>VSFRQKRTRIPLLAMTVTALAAAVCGVTTAPAATGAEVAVPLSVGAAAGNATPIPGYVIQSSAQVSDDSAVSKPGFPTSGWYPVSSRSTVYAGLLQNGKYADPFYSTNMQNVPAAQFSVPWWYRTDLNVDDTSSRTYLDFSGVLSKADVWVNGTKVATKDQVNGAYTRHDLDITAQVHTGVNSVAFKVYPNDPNRDLSMGWIDWAQTPPDQNMGIVRDVLVRRSGAVALRSAHVIQKLNSALDHADLTVKADVRNDSANAVQTTVAGTVAGKPISQTVSLAAKERKTVTFPLVGLDRPNVWWPAGMGGQHRYDLDLTASVGGTPSDAAKSKFGVRDVKATLNSSGGRQYSVNGKPLLIRGGGYTPDLFLRWNETAAADKLKYVLNLGLNTVRLEGHIEPDEFFDIADDLGVLTMPGWECCDKWEGQVNGEEKGEPWVESDYPIAKASMFSEAERLRDHPSVISFHIGSAFAPDRRIEQGYLDAMKAADFLLPVIPAASARPSPITGASGMKMNGPYDYVPPVYWYDKSQKDRGGAWSFNSETSAGVDIPTMDTLKRMMSASELDTMWKNPSAKQYHRSSSDTFGNLKLFGDALTKRYGASANLNDFVRKAQLSQYENVRAEFESHSRNYTDSTNPSTGLIYWMLNSPWTSLHWQLFDAYMDQNGAYYGAKKANEPLHIQYSHDNRSVVVINQTSNAVSGLTATTKLYNLDGTEKYSNTKTGLSVGALGAKATAVTVPAVSGLSTTYLAKNVLTDSSGKEVSRNVYWLSTKADTLNWGGSDWYYTPQSAF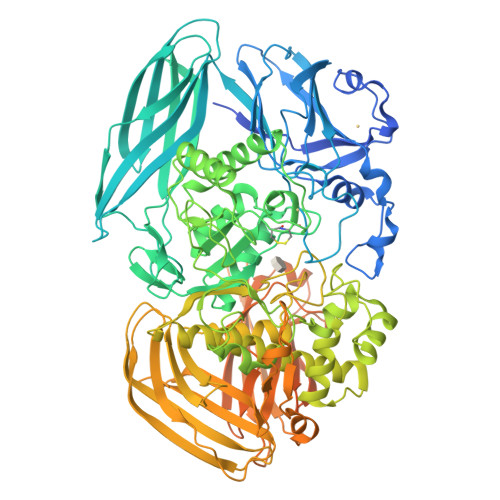ADLSGLNNLGQSAVGATANSVAGADGTTTTTVTLKNTSGGRLPAFYVDSKVVDSAGKPVLPVEWNANAVSLWPGETTTLTAKYRTADLKGSKPSVRISGWNTGTQTVPADGSGPGPSDPVDYQAEDATIVQGAVESNHAGYTGTGFVNYDNVAGSSVEWTVTVPSAGTYDVVVRYANGTTTSRPLDFSVNGSISASGVAFGSTGTWPAWTTKTVRVTLAAGVNKIKAVATTANGGPNVDKITL[2x]> EQQRFPQRYIELAIVVDHGMYTKYSSNFKKIRKRVHQMVSNINEMCRPLNIAITLALLDVWSEKDFITVQADAPTTAGLFGDWRERVLLKKKNHDHAQLLTDTNFARNTIGW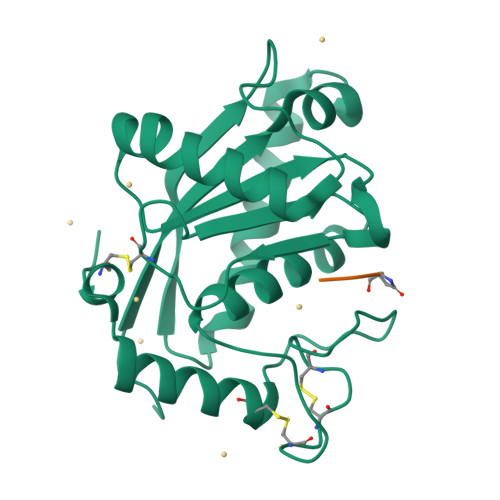AYVGRMCDEKYSVAVVKDHSSKVFMVAVTMTHELGHNLGMEHDDKDKCKCDTCIMSAVISDKQSKLFSDCSKDYYQTFLTNDNPQCILNAP;> QKW>[2x]MSGLKKFFPYSTNVLKGAAADIALPSLAGKTVFFYFSASWCPPCRAFTPQLIDFYKAHAEKKNFEVMLISWDESAEDFKDYYAKMPWLALPFEDRKGMEFLTTGFDVKSIPTLVGVEADS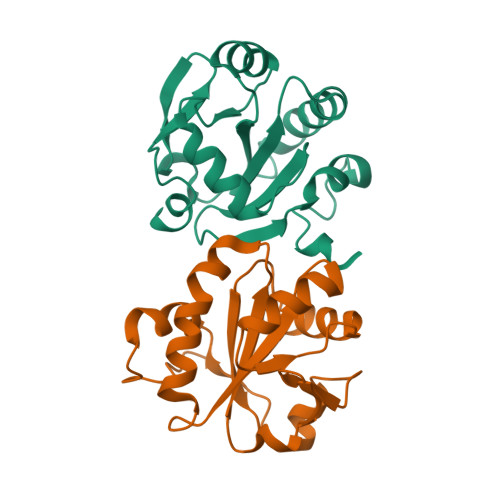GNIITTQARTMVVKDPEAKDFPWPNVEAKK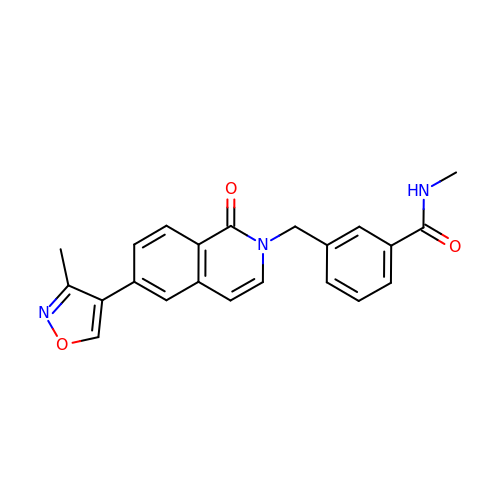~{N}-methyl-3-[[6-(3-methyl-1,2-oxazol-4-yl)-1-oxidanylidene-isoquinolin-2-yl]methyl]benzamide | C22 H19 N3 O3 | MESNOQPYPMFBSZ-UHFFFAOYSA-N>MNNNLQRDAIAAAIDVLNEERVIAYPTEAVFGVGCDPDSETAVMRLLELKQRPVDKGLILIAANYEQLKPYIDDTMLTDVQRETIFSRWPGPVTFVFPAPATTPRWLTGRFDSLAVRVTDHPLVVALCQAYGKPLVSTSANLSGLPPCRTVD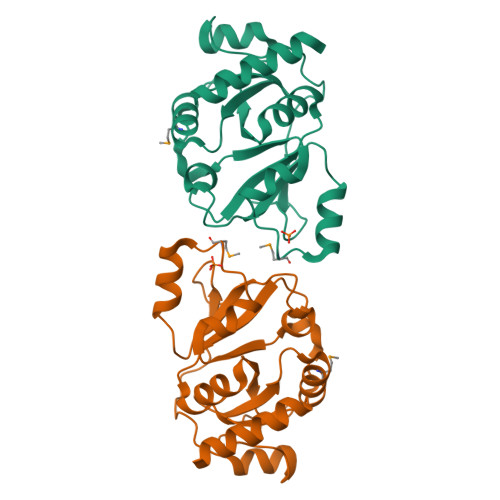EVRAQFGAAFPVVPGETGGRLNPSEIRDALTGELFR[2x]> MTHGAVKTYGIRLRVWGDYACFTRPEMKVERVSYDVMPPSAARGILEAIHWKPAIRWIVDRIHVLRPIVFDNVRRNEVSSKIPKPNPATAMRDRKPLYFLVDDGSNRQQRAATLLRNVDYVIEAHFELTDKAGAEDNAGKHLDIFRRRARAGQSFQQPCLGCREFPASFELLEGDVPLSCYAGEKRDLGYMLLDIDFERDMTPLFFKAVMEDGVITPPSRTSPEVRA;>MTAIANRYEFVLLFDVENGNPNGDPDAGNMPRIDPETGHGLVTDVCLKRKIRNHVALTKEGAERFNIYIQEKAILNETHERAYTACDLKPEPKKLPKKVEDAKRVTDWMCTNFYDIRTFGAVMTTEVNCGQVRGPVQMAFARSVEPVVPQEVSITRMAVTTKAEAEKQQGDNRTMGRKHIVPYGLYVAHGFISAPLAEKTGFSDEDLTLFWDALVNMFEHDRSAARGLMSSRKLIVFKHQNRLGNAPAHKLFDLVKVSRAEGSSGPARSFADYAVTVGQAPEGVEVKEML[7x];> MILQALHGYYQRMSADPDAGMPPYGTSMENISFALVLDAKGTLRGIEDLREQEGKKLRPRKMLVPIAEKKGNGIKPNFLWENTSYILGVDAKGKQERTDKCHAAFIAHIKAYCDTADQDLAAVLQFLEHGEKDLSAFPVSEEVIGSNIVFRIEGEPGFVHERPAARQAWANCLNRR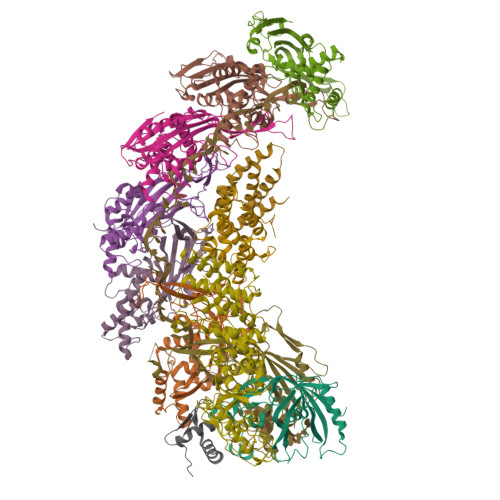EQGLCGQCLITGERQKPIAQLHPSIKGGRDGVRGAQAVASIVSFNNTAFESYGKEQSINAPVSQEAAFSYVTALNYLLNPSNRQKVTIADATVVFWAERSSPAEDIFAGMFDPPSTTAKPESSNGTPPEDSEEGSQPDTARDDPHAAARMHDLLVAIRSGKRATDIMPDMDESVRFHVLGLSPNAARLSVRFWEVDTVGHMLDKVGRHYRELEIIPQFNNEQEFPSLSTLLRQTAVLNKTENISPVLAGGLFRAMLTGGPYPQSLLPAVLGRIRAEHARPEDKSRYRLEVVTYYRAALIKAYLIRNRKLEVPVSLDPARTDRPYLLGRLFAVLEKAQEDAVPGANATIKDRYLASASANPGQVFHMLLKNASNHTAKLRKDPERKGSAIHYEIMMQEIIDNISDFPVTMSSDEQGLFMIGYYHQRKALFTKKNKEN;>VSLDPARTDRPYLLGRLFAVLEKAQEDAVPGANATIKDRYLASASANPGQVFHMLLKNASNHTAKLRKDPERKGSAIHYEIMMQEIIDNISDFPVTMSSDEQGLFMIGYYHQRKALFTKKNKEN[2x];> MDNKITPADEEKIREWLNCEEASVDNDGDVWVAVPMTGHWLSDEQKAKYIEWRGDET>GSHMVTAITNREREAVLRIEFPNVDVTDIDFDLFQARESTDKPLDVAAAIAYRLLLGSGLPQKFGCSDEVLLNFILQCRKKYRNVPYHNFYHVVDVCQTIYTFLYRGNVYEKLTELECFVLLITALVHDLDHMGLNNSFYLKTESPLGILSSASGNKSVLEVHHCNLAVEILSDPESDVFGGLEGAERTLAFRSMIDCVLATDMARHSEFLEKYLELMKTSYNVDDSDHRQMTMDVLMKAGDISNVTKPFDISRQWAM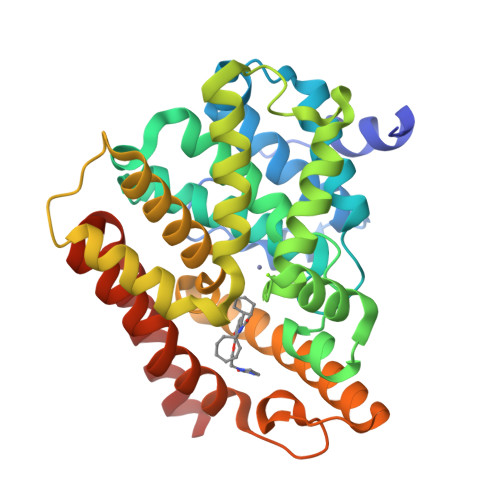AVTEEFYRQGDMEKERGVEVLPMFDRSKNMELAKGQIGFIDFVAAPFFQKIVDACLQGMQWTVDRTKSNRAQWERVLEA[2x]> CHNNSAPNYQYFPNMYESVAYEPYTEAKIFKGGKEGQLPVEGTINRGFEPYEYENSTAGYELAKANLKSPLTEEEKNSGKGKELFEIYCISCHGAAGNGKGKL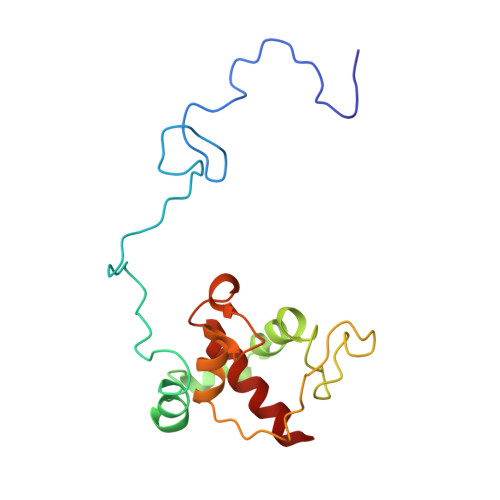VEREKFLGVPSYKDREITEGSIFHVETYGLNAMGSHANQLSAHERWLVADYVLKLKSQL>[2x]ASLTEIEHLVQSVCKSYRETCQLRLEDLLRQRSNIFSREEV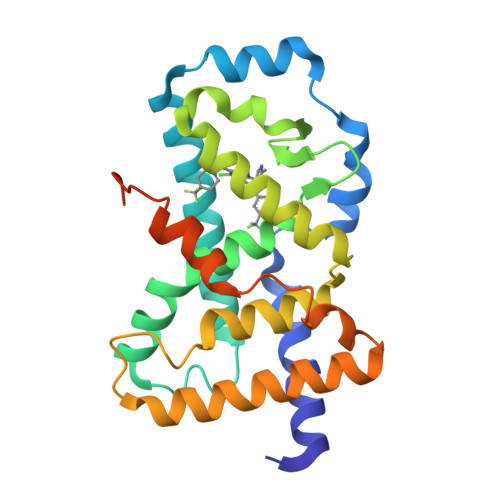TGYQRKSMWEMWERCAHHLTEAIQYVVEFAKRLSGFMELCQNDQIVLLKAGAMEVVLVRMCRAYNADNRTVFFEGKYGGMELFRALGCSELISSIFDFSHSLSALHFSEDEIALYTALVLINAHRPGLQEKRKVEQLQYNLELAFHHHLCKTHRQSILAKLPPKGKLRSLCSQHVERLQIFQHLHPIVVQAAFPPLYKELFS>[22x]MDADKIVFKVNNQVVSLKPEIIVDQHEYKYPAIKDLKKPCITLGKAPDLNKAYKSVLSGMSAAKLDPDDVCSYLAAAMQFFEGTCPEDWTSYGIVIARKGDKITPGSLVEIKRTDVEGNWALTGGMELTRDPTVPEHASLVGLLLSLYRLSKISGQNTGNYKTNIADRIEQIFETAPFVKIVEHHTLMTTHKMCANWSTIPNFRFLAGTYDMFFSRIEHLYSAIRVGTVVTAYEDCSGLVSFTGFIKQI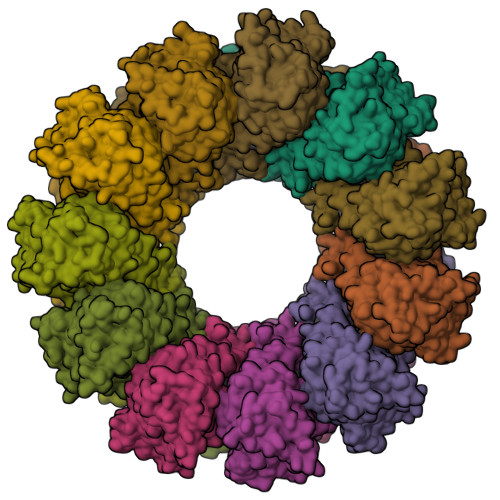NLTAREAILYFFHKNFEEEIRRMFEPGQETAVPHSYFIHFRSLGLSGKSPYSSNAVGHVFNLIHFVGCYMGQVRSLNATVIAACAPHEMSVLGGYLGEEFFGKGTFERRFFRDEKELQEYEAAELTKTDVALADDGTVNSDDEDYFSGETRSPEAVYTRIMMNGGRLKRSHIRRYVSVSSNHQARPNSFAEFLNKTYSSDS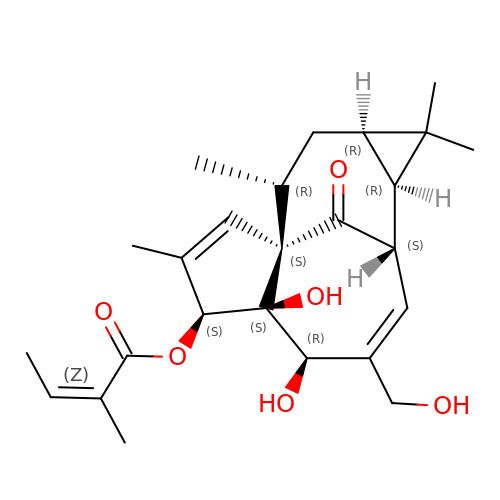ingenol-3-angelate | C25 H34 O6 | VDJHFHXMUKFKET-WDUFCVPESA-N>[2x]MALGPLVTGL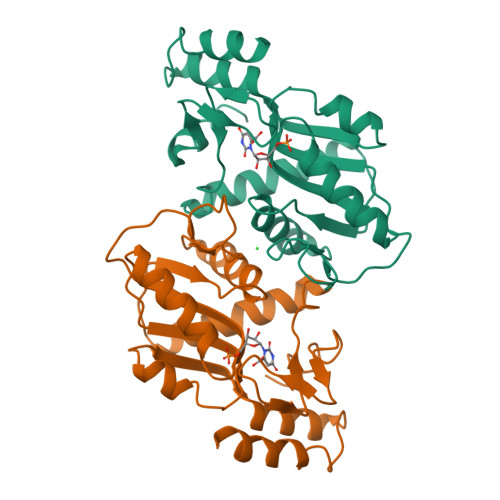YDVQAFKFGDFVLKSGLSSPIYIDLRGIVSRPRLLSQVADILFQTAQNAGISFDTVCGVPYTALPLATVICSTNQIPMLIRRKETKDYGTKRLVEGTINPGETCLIIEDVVTSGSSVLETVEVLQKEGLKVTDAIVLLDREQGGKDKLQAHGIRLHSVCTLSKMLEILEQQKKVDAETVGRVKRFIQEAHHHHHH>MPNIKIFSGSSHQDLSQKIADRLGLELGKVVTKKFSNQETCVTIGESVRGEDVYIVQSGCGEINDNLMELLIMINACKIASASRVTAVIPCFPYARQDKKDKSRAPISAKLVANMLSVAGADHIITMDLHASQIQGFFDIPVDNLYAEPAVLKWIRENISEWRNCTIVSPDAGGAKRVTSIADRLNVDFALIHKERKKANEVDRMVLVGDVKDRVAILVDDMADTCGTICHAADKLLSAGATRVYAILTHGIFSGPAISRINNACFEAVVVTNTIPQEDKMKHCSKIQVIDISMILAEAIRRTHNGESVSYLFSHVPLLEHHHHHH[2x]

PRPP is formed from ATP and D-ribose-5-phosphate (R5P) by the phosphoribosyl pyrophosphate synthetases (PRSs). The human PRS family, which has 3 isoforms (hPRS1, hPRS2 and hPRS3), belongs to the class I PRSs that requires divalent metal ions such as Mg2+ as the activator, inorganic phosphate ion for activity, and ATP or dATP as the diphosphoryl donor. Due to the important role of PRPP in the nucleotide metabolic process, the stability of PRPP content is essential for cell physiology and is predominantly controlled by hPRS1, the ubiquitously expressed human PRPP synthetase. Mutations in hPRS1 affect vital cell functions and are related to many diseases and disorders.

We determined the crystal structures of the E43T, D65N, A87T, M115T and Q133P mutations at a resolution of 3.0 Å, 2.14 Å, 3.3 Å, 2.11 Å and 2.74 Å, respectively, with 2 molecules in each asymmetric unit. Overall, the structures of all the five structures are highly similar to that of the wild type PRS1 with RMSD listed in S2 Table. In the low resolution E43T structure, the Glu43 replaced by Thr43 might destroy the hydrogen bond interaction between Glu43 and Ser103, which might reduce the restraint of both the ATP binding motif β2–3 and the catalytic flexible loop. It is confirmed by the MD simulation. The E43T mutant affects both the ATP binding motif and the catalytic flexible loop and therefore displays as low activity.> MSSISLKEIIPPQPSTQRNFTTHLSYDPTTNAIAYPCGKSAFVRCLDDGDSKVPPVVQFTGHGSSVVTTVKFSPIKGSQYLCSGDESGKVIVWGWTFDKESNSVEVNVKSEFQVLAGPISDISWDFEGRRLCVVGEGRDNFGVFISWDSGNSLGEVSGHSQRINACHLKQSRPMRSMTVGDDGSVVFYQGPPFKFSASDRTHHKQGSFVRDVEFSPDSGEFVITVGSDRKISCFDGKSGEFLKYIEDDQEPVQGGIFALSWLDSQKFATVGADATIRVWDVTTSKCVQKWTLDKQQLGNQQVGVVATGNGRIISLSLDGTLNFYELGHDEVLKTISGHNKGITALTVNPLISGSYDGRIMEWSSSSMHQDHSNLIVSLDNSKAQEYSSISWDDTLKVNGITKHEFGSQPKVASANNDGFTAVLTNDDDLLILQSFTGDIIKSVRLNSPGSAVSLSQNYVAVGLEEGNTIQVFKLSDLEVSFDLKTPLRAKPSYISISPSETYIAAGDVMGKILLYDLQSREVKTSRWAFRTSKINAISWKPAEKGANEEEIEEDLVATGSLDTNIFIYSVKRPMKIIKALNAHKDGVNN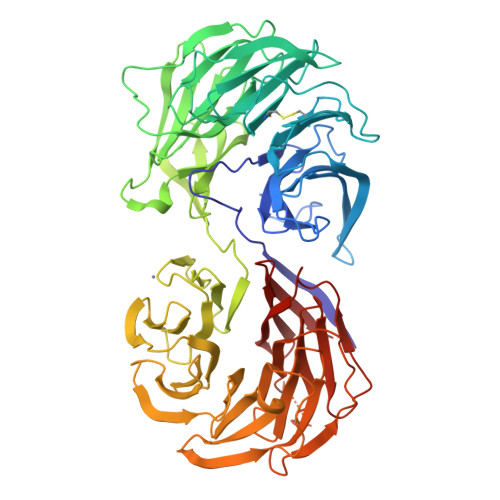LLWETPSTLVSSGADACIKRWNVVLE> GWPHSIESSNDWNVEKRSIRDVPVVRLPADSPIPERGDLSCRMHTCFDVYRCGFNPKNKIKVYIYALKKYVDDFGVSVSNTISREYNELLMAISDSDYYTDDINRACLFVPSIDVLNQNTLRIKETAQAMAQLSRWDRGTNHLLFNMLPGGPPDYNTALDVPRDRALLAGGGFSTWTYRQGYDVSIPVYSPLSAEVDLPEKGPGP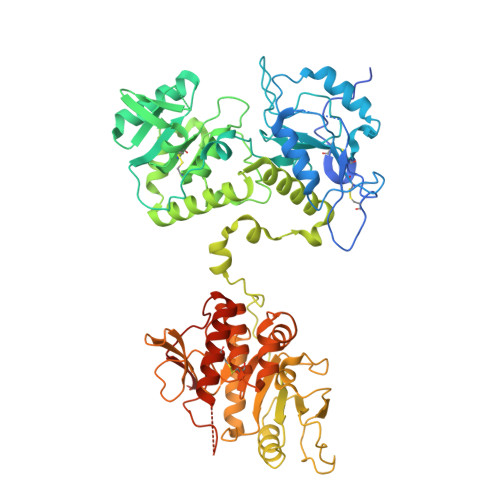RQYFLLSSQVGLHPEYREDLEALQVKHGESVLVLDKCTNLSEGVLSVRKRCHKHQVFDYPQVLQEATFCVVLRGARLGQAVLSDVLQAGCVPVVIADSYILPFSEVLDWKRASVVVPEEKMSDVYSILQSIPQRQIEEMQRQARWFWEAYFQSIKAIALATLQIINDRIYPYAAISYEEWNDPPAVKWGSVSNPLFLPLIPPQSQGFTAIVLTYDRVESLFRVITEVSKVPSLSKLLVVWNNQNKNPPEDSLWPKIRVPLKVVRTAENKLSNRFFPYDEIETEAVLAIDDDIIMLTSDELQFGYEVWREFPDRLVGYPGRLHLWDHEMNKWKYESEWTNEVSMVLTGAAFYHKYFNYLYTYKMPGDIKNWVDAHMNCEDIAMNFLVANVTGKAVIKVTPRKKFKCPECTAIDGLSLDQTHMVERSECINKFASVFGTMPLKVVEHRADPVLYKDDFPEKLKSFPNIGSL methyl (2E,6E)-9-[(2R)-3,3-dimethyloxiran-2-yl]-3,7-dimethylnona-2,6-dienoate 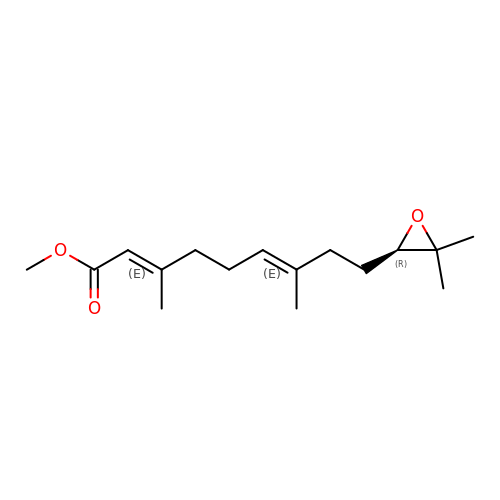| C16 H26 O3 | QVJMXSGZTCGLHZ-HONBPKQLSA-N> MSRNPSNSDAAHAFWSTQPVPQTEDETEKIVFAGPMDEPKTVADIPEEPYPIASTFEWWTPNMEAADDIHAIYELLRDNYVEDDDSMFRFNYSEEFLQWALCPPSYIPDWHVAVRRKADKKLLAFIAGVPVTLRMGTPKYMKVKAQEKGQEEEAAKYDAPRHICEINFLCVHKQLREKRLAPILIKEVTRRVNRTNVWQAVYTAGVLLPTPYASGQYFHRSLNPEKLVEIRFSGIPAQYQKFQNPMAMLKRNYQL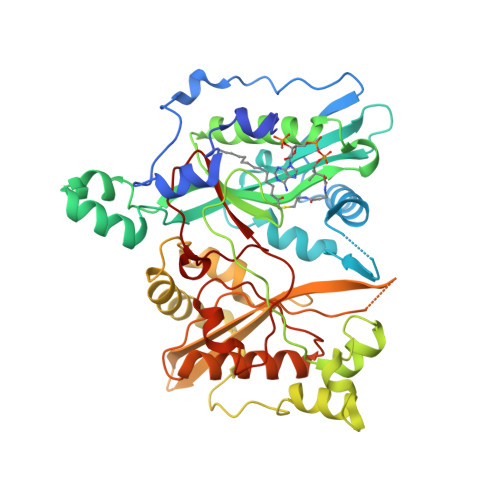PNAPKNSGLREMKPSDVPQVRRILMNYLDNFDVGPVFSDAEISHYLLPRDGVVFTYVVENDKKVTDFFSFYRIPSTVIGNSNYNILNAAYVHYYAATSMPLHQLILDLLIVAHSRGFDVCNMVEILDNRSFVEQLKFGAGDGHLRYYFYNWAYPKIKPSQVALVML> MSKNRSSLQSGPLNSELLEEQKQEIYEAFSLFDMNNDGFLDYHELKVAMKALGFELPKREIL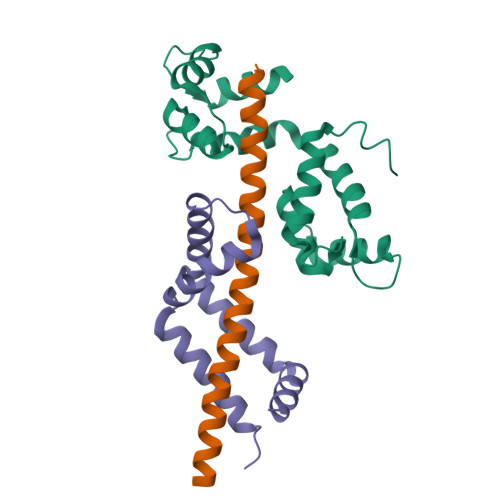DLIDEYDSEGRHLMKYDDFYIVMGEKILKRDPLDEIKRAFQLFDDDHTGKISIKNLRRVAKELGETLTDEELRAMIEEFDLDGDGEINENEFIAICTDS;> GSEANYRKDFIDTMTRELYDAFLHERLYLIYMDSRAELKRNSTLKKKFFEKWQAS;> MTMDTAQLKSQIQQYLVESGNYELISNELKARLLQEGWVDKVKDLTKSEMNINESTNFTQILSTVEPKALEMVSDSTRETVLKQIREFLEEIVDTQ>MTVTLNMEKYNFLG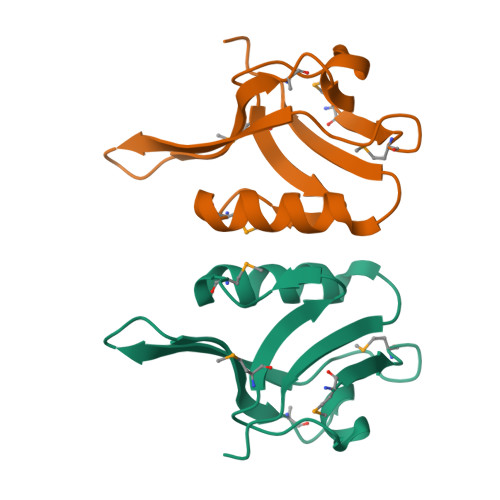ISIVGQSNERGDGGIYIGSIMKGGAVAADGRIEPGDMLLQVNDINFENMSNDDAVRVLRDIVHKPGPIVLTVAKCWD[2x]>GKITLYEDRGFQGRHYECSSDHPNLQPYLSRCNSASVDSGCWMLYEQPNYSGLQYFLRRGDYADHQQWMGLSDSVRSCRLIPHSGSHRIRLYERED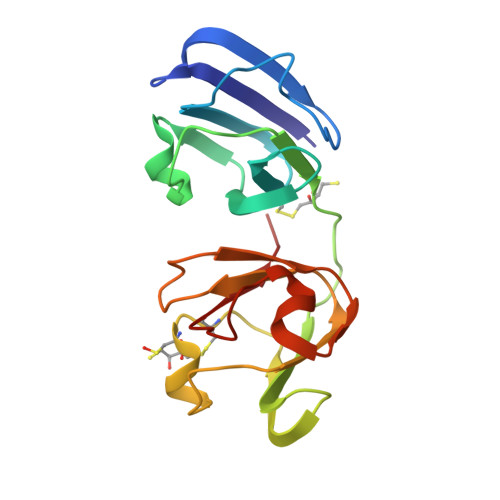YRGQMIEFTEDCSCLQDRFRFNEIHSLNVLEGSWVLYELSNYRGRQYLLMPGDYRRYQDWGATNARVGSLRRVID[2x]>MRVLGIDPGLANLGLGLVEGDVRRAKHLYHVCLTTESAWLMPRRLQYLHEELTRLLTEYRPDAVAIEDQILRRQADVAFKVGQAFGVVQLACAQAGVPIHAYGPMQVKKSLVGTGRADKEQVIYMVKASLGIRELFNNHAADALALALTHLAHAPMQERSERLAAAGRAARTGDAPLRR[2x]

D. radiodurans encodes two putative HJ resolvase (HJR) homologs: RuvC (DrRuvC) and YqgF (DrYqgF). The widespread bacterial RuvC and YqgF are evolutionarily connected, and both possess a canonical RNase H-like fold, including five β-strands (β1 to β5) and three α-helices (α1 to α3). The apo structures of RuvC and YqgF from D. radiodurans (DrRuvC and DrYqgF, respectively) were determined by X-ray crystallography. To sum up, our study showed that DrRucC might act as a major HJR in D. radiodurans, while DrYqgF might play certain roles in RNA metabolism.

The refined DrRuvC model contains two monomer molecules in an asymmetric unit. Each monomer is comprised of five β-strands (β1 to β5), and these strands are sandwiched by five α-helices (α1, α2, α3a, α3b, and α3), forming a canonical Rossman fold. The DrRuvC dimer structure superimposed well with the TtRuvC structure (the root-mean-square deviation [RMSD] value for 258 Cα atoms is 1.665 Å), EcRuvC structure (the RMSD value for 268 Cα atoms is 1.933 Å), and PaRuvC structure (the RMSD value for 280 Cα atoms is 2.111 Å), in agreement with their high conservations of amino acid sequences. The two monomers of DrRuvC are bound together through interactions, mainly between α2, involving both polar (Q83 and Q89) and hydrophobic interactions (F79, F85, V87, and L90). Interestingly, the DrRuvC homodimer exhibits distinct asymmetry in residues 73 to 83 spanning the dimer interface, which is also observed in the TtRuvC apo structure. The high-temperature structure factor values indicate that the area around the DrRuvC residues 73 to 83 is not rigid and might undergo a disorder-to-order transition upon HJ substrate binding. Although the crystal condition contains 0.2 M MgCl2, only weak metal ion density was observed in the DrRuvC structure. The fourth catalytic residue of RuvC, which is also located at α3 and is usually glutamate, is replaced by histidine in DrRuvC and TtRuvC. Replacement by alanine of the putative catalytic residues in DrRuvC (D7A, E67A, H139A, and D142A) abolished its HJR activity. DrRuvC could preferentially cleave HJ at the consensus 5′-(G/C)TC↓(G/C)-3′ sequence and could prefer using Mn2+ for catalysis in vitro, which would be different from the preferences of the other previously characterized RuvCs.> MDGVHDLAGVQGFGKVPHTVDADIGPTFHAEWEHLPYSLMFAGVAELGAFSVDEVRYVVERMEPRHYMMTPYYER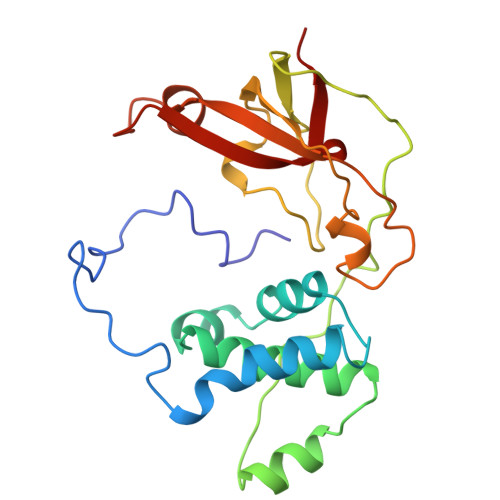YVIGVATLMVEKGILTQDELESLAGGPFPLSRPSESEGRPAPVETTTFEVGQRVRVRDEYVPGHIRMPAYCRGRVGTISHRTTEKWPFPDAIGHGRNDAGEEPTYHVKFAAEELFGSDTDGGSVVVDLFEGYLEPAA> MGSSHHHHHHGTGSYITSLYKKAGWMGSNEAQVKKESIGEIMGKLMQGEIGDEELSKRIKEIFGKRLQWGYKPTHQQQLAFNLDFIKSLKEMDMSGEIDTMNEETYELPSAFLEAAFGKTIKQSGCYFKDETTTIDEA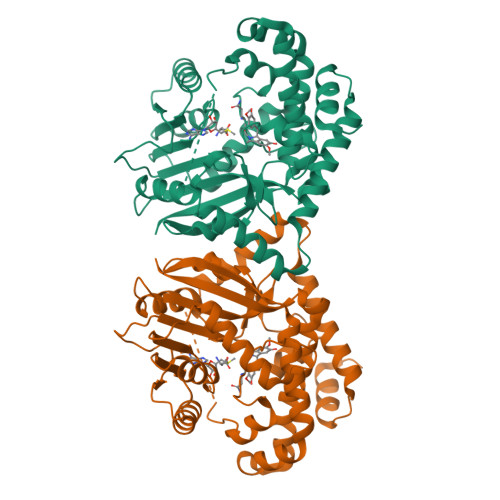EEASHELYCERAQIKDGQTVLDIGCGQGGLVLHIAQKYKNCHVTGLTNSKAQKNYILMQAEKLQLSNVDVILADVTKHESDKTYDRILVIETIAHMKNIQLFMKKLSTWMTEDSLLFVDHICHKTFSHHFEAIDEDDWYSGFIFPKGCVTILSASALLYFQDDVTILDHWVVNGMHMARSVDAWRKKLDKNMELAREILLPGLGSKEAVNGVITHIRTFCMGGYEQFSYNNGEEWMVAQMLFKKK>[2x]SNAMEIKSILIANRGEIALRALRTIKEMGKKAICVYSEADKDALYLKYADASICIGKARSSESYLNIPAIIAAAEIAEADAIFPGYGFLSENQNFVEICAKHNIK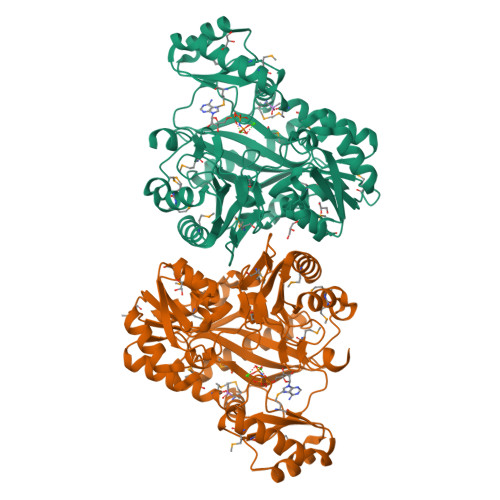FIGPSVEAMNLMSDKSKAKQVMQRAGVPVIPGSDGALAGAEAAKKLAKEIGYPVILKAAAGGGGRGMRVVENEKDLEKAYWSAESEAMTAFGDGTMYMEKYIQNPRHIEVQVIGDSFGNVIHVGERDCSMQRRHQKLIEESPAILLDEKTRTRLHETAIKAAKAIGYEGAGTFEFLVDKNLDFYFIEMNTRLQVEHCVSEMVSGIDIIEQMIKVAEGYALPSQESIKLNGHSIECRITAEDSKTFLPSPGKITKYIPPAGRNVRMESHCYQDYSVPAYYDSMIGKLVVWAEDRNKAIAKMKVALDELLISGIKTTKDFHLSMMENPDFINNNYDTNYLARH> NFGPGTELTVLPLEKTLLTESGGGTYQAGKTLSLKCQTSGFQFKTSQLDWYLWTPGHAPLWLTGLNSSSTDATEGRITSSREDNKNQIFLQIEDLGLRDSGQYHCARRVGNGDDTDKLVFGLGTRVIVEPRPAAPLSPSVFLVRDQDAVACLIRNFYPKELHVSLTSSGTLISAQSLSLAPTASG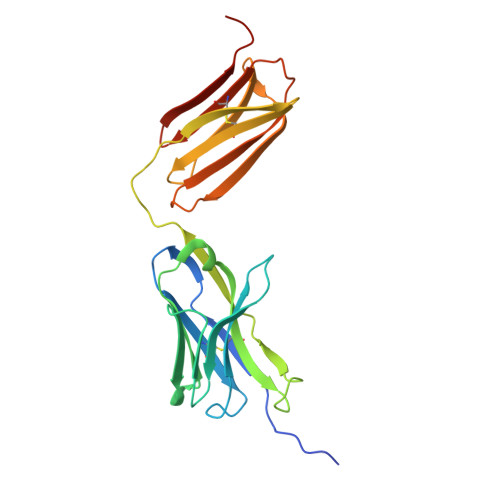TYSAIHIGRVGENDAITCSVKHLGKEIHMSHQAGSLVPR>MAPSAYALDRSSVPSGKPRLMEGAESKARAGARKIHHLKIHGFDRVFGPGTHRWQRALWFAGVVFCFGISAHQIAMHVLDYLSEPVAVRIDFVAQNELRIPEITVCPRIFQQNTIFTDMVEKQGIDKMKFLDLIDRPEYDIMAVWNLSRIFSDNVSCSAHEGSSIISGSYVDPNMSQPHLVYTTSGQCINIPASRPLIYRGVNTFVRITDSQPRNLNQVRPEAIQIYFHEHHHAHLSRYLTGLRGYIVPIANPFAFSIRFTQINYANKTDSPCVDSEEYAACVEDFIEQRIYEKAQVQCRLPYMRPKLPLCSTPTDARKIFVATDDVIQNFEKESSCKRKCEETLYIVE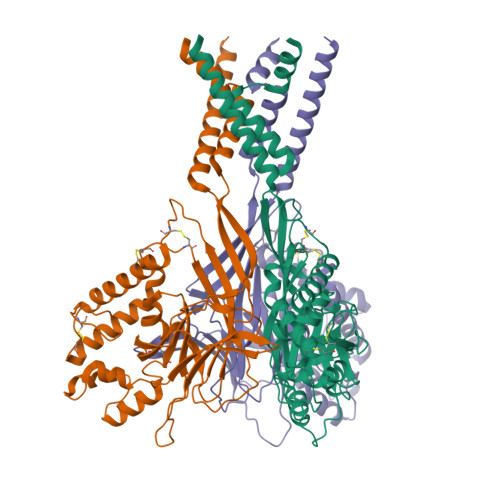FMHLFERSNISIDMSVYFAYNYIQVATEYLTYTLRGLLSDIGGVLGLFLGICILSVIEVFEVVIFSLQRVLCNEDKKQQNNE[3x]> MGSSMKLKHKRDDKMRFDIKKVLELAEKDFETAWRETRALIKDKHIDNKYPRLKPVYGKPHPVMETIERLRQAYLRMGFEEMINPVIVDEMEIYKQFGPEAMAVLDRCFYLAGLPRPDVGLGNEKVEIIKNLGIDIDEEKKERLREVLHLYKKGAIDGDDLVFEIAKALNVSNEMGLKVLETAFPEFKDLKPESTTLTLRSHMTSGWFITLSSLIKKRKLPLKLFSIDRCFRREQREDRSHLMSYHSASCVVVGEDVSVDDGKVVAEGLLAQFGFTKFKFKPDEKKSKYYTPETQTEVYAYHPKLGEWIEVATFGVYSPIALAKYNIDVPVMNLGLGVERLAMIIYGYEDVRAMVYPQFYEYRLSDRDIAGMIRVDKVPILDEFYNFANELIDICIANKDKESPCSVEVKREFNFNGERRVIKVEIFENEPNKKLLGPSVLNEVYV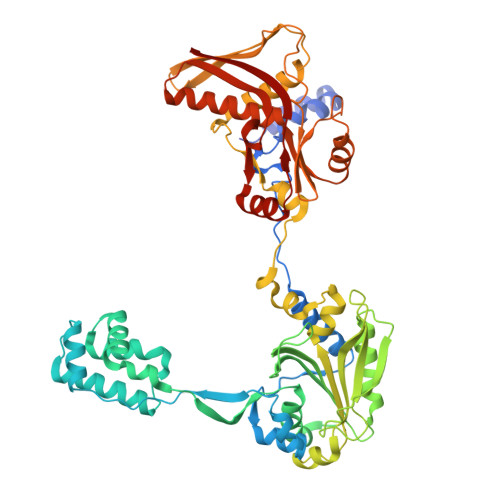YDGNIYGIPPTFEGVKEQYIPILKKAKEEGVSTNIRYIDGIIYKLVAKIEEALVSNVDEFKFRVPIVRSLSDINLKIDELALKQIMGENKVIDVRGPVFLNAKVEIK> HMASMKKKGSVVIVGRINLSGDTAYAQQTRGEEGCQETSQTGRDKNQVEGEVQIVSTATQTFLATSINGVLWTVYHGAGTRTIASPKGPVTQMYTNVDKDLVGWQAPQGSRSLTPCTCGSSDLYLVTRHADVIPVRRRGDSRGSLLSPRPISYLKGSSGGPLLCPAGHAV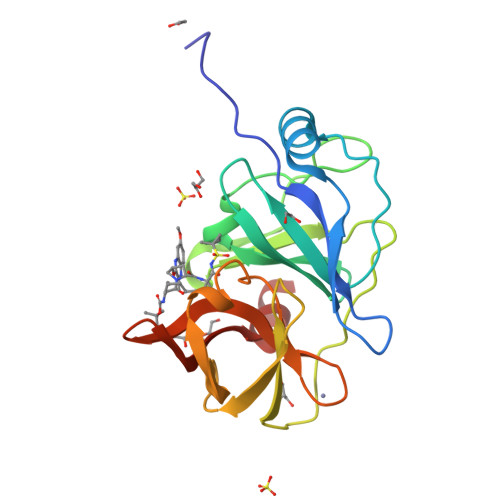GIFRAAVSTRGVAKAVAFIPVESLETTMRS> SKPQPIAAANWKCNGSQQSLSELIDLFNSTSINHDVQCVVAPRFVMIAMTKERLSHPKFVIAAQNAG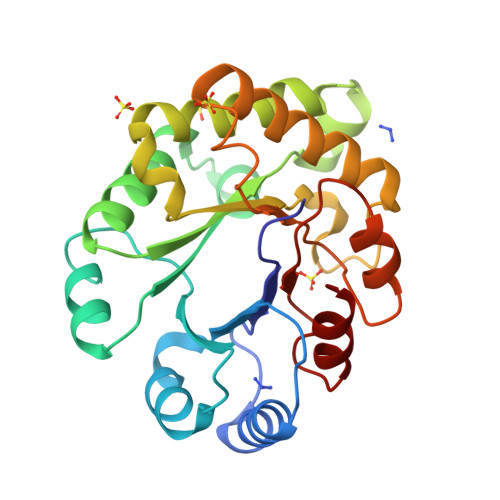NADGLASLKDFGVNWIVLGHSERRAYYGETNEIVADKVAAAVASGFMVIACIGETLQERESGRTAVVVLTQIAAIAKKLKKADWAKVVIAYEPVWAIGTGKVATPQQAQETHALIRSWVSSKIGADVAGELRILYGGSVNGKNARTLYQQRDVNGFLVGGASLKPEFVDIIKATQ>DVNLYGPGGPHTALKDIANKYSEKTGVKVNVNFGPQATWFEKAKKDADILFGASDQSALAIASDFGKDFNVSKIKPLYFREAIILTQKGNPLKIKGLKDLANKKVRIVVPEGAGKSNTSGTGVWEDMIGRTQDIKTIQNFRNNIVAFVPNSGSARKLFAQDQADAWITWIDWSKSNPDIGTAVAIEKDLVVYRTFNVIAKEGASKETQDFIAYLS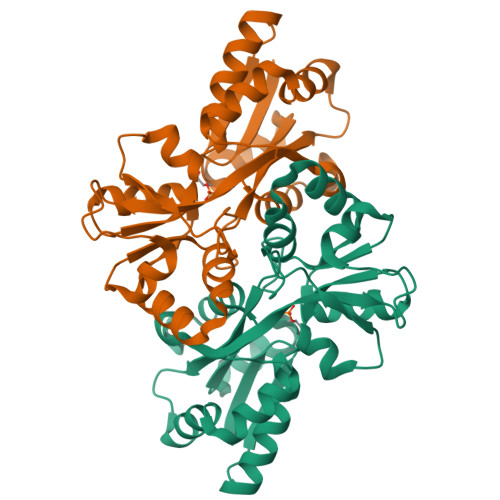SKEAKEIFKKYGWREH[2x]> GSHMSPSAQELKEQGNRLFVGRKYPEAAACYGRAITRNPLVAVYYTNRALCYL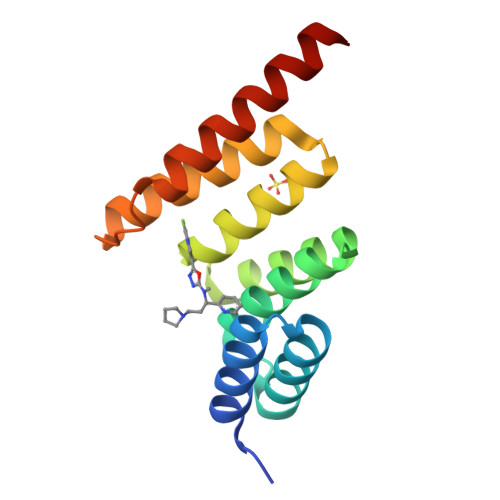KMQQHEQALADCRRALELDGQSVKAHFFLGQCQLEMESYDEAIANLQRAYSLAKEQRLNFGDDIPSALRIAKKKRWNSIEERR>[2x]HHHHHHSSGLVPRGSHMPTPSQHKDASTAQTDNQVPTGRRAQKREQTRARLITSARTLMAERGVDNVGIAEITEGANIGTGTFYNYFPDREQLLQAVAEDAFESVGIALDQVLTKLDDPAEVFAGSLRHLVRHSLEDRIWGGFFIQMGAAHPVLMRILGPRARRDLLHGLETGRFTIEDLDLATTCTFGSLIAAIQMALSADQDSNDDKDQIFAAAMLRMVGVQAAEAREIASRPLPEISPVKPQ

Here we report the crystal structures of a novel transcriptional repressor RolR and its complex with the regulator resorcinol. The RolR protomer is folded as two domains, the DNA-binding domain at N-terminal and the signal-receiving domain at C-terminal. In addition, RolR is the sole TetR-type regulator that has been identified for regulation of aromatic catabolism. RolR is an all-helix protein and each subunit is composed of 9 α helices (h1, h2, h4–h10) and two 310 helices for h3 and g1, a stretch between h1 and h2.

The crystal structure of RolR complexed with resorcinol (res-RolR) has been determined using the MAD method at 2.5 Å resolution with R factor of 0.212 and Rfree of 0.245. The structure shows a “Ω” like homo-dimer in the asymmetric unit, which is similar to those observed in other TetR structures. Two resorcinol molecules are respectively bound to the two C-domains of the RolR dimer and the resorcinol-binding pockets are identical in both monomers. The binding pocket is formed by 5 helices (helices h4–h8) of the C-terminal domain. In the binding pocket, the resorcinol molecule is located in a internal amphiphilic cavity, in which a cluster of hydrophobic residues interacts with the phenyl ring and a hydrogen bond network is bound to atoms O1 and O2 of the resorcinol molecule. A number of hydrophobic residues, including Phe107, Phe172, Leu111, Leu114 and Leu142 from helix h4–h8, are involved in contacting with the phenyl ring, while residues Asp94, Asp149, Arg145 and Arg148 interact with O1 and O2 atoms of resorcinol via a hydrogen bond network mediated by two water molecules, W1 and W2. In this network residue Asp149 directly interacts with atom O1 of resorcinol, while residues Arg148 and Asp94 interact with atom O2 of resorcinol through water molecule W2. Interestingly, these two paths are closely connected each other via hydrogen bonds among residues Asp149, Arg148 and water molecules to form a unique recognition mode (Asp149-W1-W2-Arg148-Asp94) for binding with resorcinol. The results show that the binding ability of mutant D149A to resorcinol is totally lost, while those of mutants R145A, D94A and R148A are dramatically reduced to 8.6%, 5.1% and 2.8%, respectively, in comparison with that of the wild type RolR. It indicates that the DNA-binding domain is rather rigid in res-RolR comparing with that in apo-RolR which should be unsuitable for DNA binding.> EHLAPEPAEMARLVAGTHHNPHGILGAHEYDDHTVIRAFRPHAVEVVALVGKDRFSLQHLDSGLFAVALPFVDLIDYRLQVTYEGCEPHTVADAYRFLPTLGEVDLHLFAEGRHERLWEVLGAHPRSFTTADGVVSGVSFAVWAPNAKGVSLIGEFNGWNGHEAPMRVLGPSGVWELFWPDFPCDGLYKFRVHGADGVVTDRADPFAFGTEVPPQTASRVTSSDYTWGDDDWMAGRALRNPVNEAMSTYEVHLGSWRPGLSYRQLARELTDYIVDQGFTHVELLPVAEHPFAGSWGYQVTSYYAPTSRFGTPDDFRALVDALHQAGIGVIVDWVPAHFPKDAWALGRFDGTPLYEHSDPKRGEQLDWGTYVFDFGRPEVRNFLVANALYWLQEFHIDGLRVDAVASMLYLDYSRPEGGWTPNVHGGRENLEAVQFLQEMNATAHKVAPGIVTIAEESTPWSGVTRPTNIGGLGFSMKWNMGWMHDTLDYVSRDPVYRSYHHHEMTFSMLYAFSENYVLPLSHDEVVHGKGTLWGRMPGNNHVKAAGLRSLLAYQWAHPGKQLLFMGQEFGQRAEWSEQRGLDWFQLDENGFSNGIQRLVRDINDIYRCHPALWSLDTTPEGYSWIDANDSANNVLSFMRYGSDGSVLACVFNFAGAEHRDYRLGLPRAGRWREVLNTDATIYHGSGIGNLGGVDATD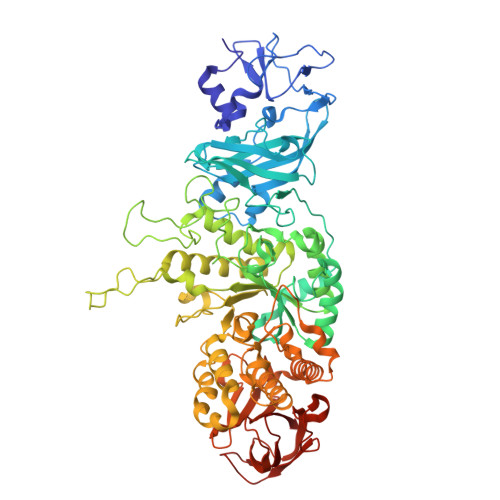DPWHGRPASAVLVLPPTSALWLTPA> MAVTATILASSGGAKTTTAEADKFDYTVEQFADLQILRYKVPEFETLTLKQKELVYYLTQAALEGRDILFDQNGKYNLRIRRMLEAVYTNYKGDKSAPDFKNMEVYLKRVWFSNGIHHHYGMEKFVPGFSQDFLKQAVLGTDAQLLPLSEGQTAEQLSDELFPVMFDPAILAKRVNQADGEDLVLTSASNYYDGVTQQEAESFYGAMKDPKDETPVSYGLNSRLVKEDGKIQEKVWKVGGLYTQAIEKIVYWLKKAETVAENDAQKAVISKLIQFYETGSLKDFDEYAILWVKDLDSRIDFVNGFTESYGDPLGVKASWESLVNFKDLDATHRTEIISSNAQWFEDHSPVDKSFKKEKVKGVSAKVITAAILAG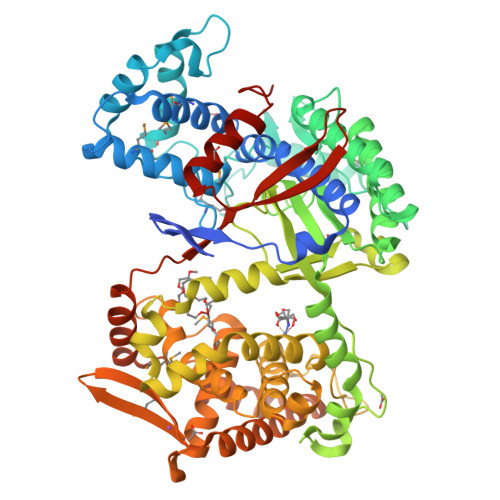DLYPATAIGINLPNANWIRAHHGSKSVTIGNITDAYNKAAHGNGFNEEFVSNDEERQRIDQYGDLTGELHTDLHESLGHGSGKLLPGVDPDALKAYGSTIEEARADLFGLYYVADPKLVELKLVPDAEAYKAEYYTFLMNGLMTQLVRIEPGNNIEEAHMRNRQLIARWVFEKGAPDKVVEMVKKDGKTYVVVNDYEKVRQLFGELLAEIQRIKSTGDFEGARTLVENYAVKVDPALHAEVLARYKKLNLAPYKGFINPVYELVTDKDGNITDVTVSYNEDYVEQMLRYSKDYSPLPSVNNLEHHHHHH> KYSKRIAWMKTTICDSLQLKDMIVEESFQYEKNKNLLEQFLSGEGLNKIFAYYQVQEQAQNDDIKDTGAQDPVLFFTTGDLEKIQDKAVWFLRITNPADDKKKASQQDGNDNDIIFGEITPNTVPMLNALMESVYSRQIDHIITEKIQFWGVAEEEQVLEFQQHSNKFSSEVREAINLMSPGTEHFKLDYEAISGLSESEKMQHYEMKFNEWINLISSQLNDDSEVRKDEKDAGPATELIYWRSRMQKITNWSEQLKSKDFQIVKASLQRHKNHDNQRPRGDESLSKLMMEYNRLDLLLTDKLNEAKDNVKYLTTLEKFIEPLYNGTPQQIIDTLPALMNAIKMIHTIARFYNTTDKMTGLFIKITNQMIKNCKDRILNKKDNGDNPSLYKMIWEQDPAELIEVLGSCIKLYCEYKKCYNDTKEKVADMPKGKTFDFSDAQIFGKFDTFVRRLQKLIEIFSNIQQFNALAKHNLEGMDVLTNKFKKIIDDFKKKGHNLLDTANNKFDRDWVEFNVEISHLDGELQNFIDNNFNRFRNIEYSLKLLHKFQSTIKRDSLKHNLTSRYNAILHNYATELDTIQRVFQDQKSNPPLVRNMPPEAGKIIWARHLFQKITGPINIFPENVINSTEIRRYYGSYNTLGKQLTIYEMWFYQDWVNKIEQSKAALQATLIVRHDENKKLYVNFDLEIMQLIREAKCLDRQGIEIPESARIILLQEDKFKTYYNELLYALKEYERINSKIKPICKNLLLPHIEDLDLKLRPGMVTLTWTSMNIESYLYYVHQGLKKLEQLIINVNDIIENRIENNLKTVSKVVLVHLPQDTKPLSLDSFVQLQEEYINSKTDFLTSKNVEVERAVDDLLQTIMLYPLDPHVDPVLPEETKRIKRYYFWYFYQALLNSTQNSLNAMKYRVCGKKIPGANTLQNLKPFFQVEVQLNGDKVTLNPSLQEIQKSINRAATAVLRCSKHLYNWDQQNKDSTDKATFYDMIACDKEIVKVILLLTGSIQGTKNKVNEFLSGFTKFEWLCKESIQESIKKFSKNGPTLQNYEDQLKKFSQIEEEIEKIVPTYKIGAMELMTHNICTSLSTWAKEWKLQYSQDLHKRARQLLDSLTEQTKMLSTKLSKPVKDIDSLGYVMETLEQIRKEQAEIDMKFNPVQEMYSLLDNYLPGGITDKDEMDARSLLRRNWDILIQQAEIKGKEYQHKQAIYLKELKQSIKDFTNQVSIFRRDYEKNGPMVEGISPAEAMERLRRFEDEYDVKYQMYKINARGENLFGLQNQKYPELEKTDAEIKNLNKLYNLYDSVIKNIQQFKEKSWQDVSKDDLAKMEEDAGKYGEQCSRLPKDLKEWQAYRDLKNYIDSLREQLPLIISLKKPSIMPRHWEKIKEITNTKLNYENPDQFYIEEIMGAKLLDFREDIEDITESADKQLKIRTGLDEINLYWNDMQFQFGIWGKRDVPCMLNGLIVGTILERLEEDQLQLSTFNSQRHVTPFKAEVENLIRTFSDVNDTLDMWVKVQKLWTSLEPVFTGGDIARQMPLQAKQFQGIDKNWMKIMEKAVETKKVIPCCQNDMLKDFLPDLNRKLEDCQKMLEAYLEGKRKKFPRFYFVSNPTLLKILSQGSEPTSIQEDFEKLFDAITKVTFESAKDKKNPALKQITQIQQVIGRNEENISLTGYYVKCEGNIEDWLKKLEQNMQQTLKDIASAAAQQVFQVGLKEFVSSQASQIALLGLQILWTSKVNEGLERLSRNERNAMDIKRNEIKEHMNILSSMCLEDLNGAVERTKVETLVTIQVHQKDISMDLKCKDVNDFEWQKQTRIAWKTDIDECIISITDWDSPYSYEFLGAKERLCITPLTDRCYITLAQAMSMYYGGAPAGPAGTGKTETVKDLGRTLGVFVVVTNCSDQHRYRDMAKIFKGLVQSGLWGCFDEFNRIDLEVLSVVAMQVESITTARKQHMKKFMFPEEEIEIELIPTVSYFITMNPGYAGRQELPENLKVLFRGVSMMVPDREIIIKVKLASVGYLQIDLLAKKFNVLYRLCEEQLSKQRHYDFGLRNILSVLRTAGNTKRQEIKSDEEMLLMRSLRDMNLSKLVADDIPLFNGLLADIFPKLKEVPKKLYPDVEKKIPEEINAESYLINTPSFQLKIIQLYETCLVRHGFMLVGPTGSGKSTIMKILTEVLTKLGSPHKIVIMNPKAITAEQMYGVKSEISDDWIPGVFSTIWAKSNNRALKHTTWITCDGPVDAIWIENLNTVLDDNKILTLANGERIAMTENCKVVFEVENLNNASPATVSRCGQVYVSPTDLGYEAVIEGWIRNRKASGRAEESDKLGNILRKYLINMRFIELQSKECKEPMMDTSPVISVINILNLLTGCLQYFVQTQRTLSEQEYEKFIVYSMAWAIGGIYEAQDRVRFHELLLAKNAPIPQKGKENETVFDYYVSQDYLDWKICSPEEWVPPQSLQFSQLLLPTLDSFRAEMLLNFILTQPKSHTCSNSALLIGGSGTAKTSSVLLYCNKFDPQKMLFKRTNFSSATSPFMFQSTIEAECDFKVGKEFAPPGNKMMTIFIDDMSMPFVNKWGDQITLELVRQLIETGGFYMLDKTQRGNQRKMKNLQYIGAMNHPGGGRNDIPNRLKRQFFIFNMILPLSIEGIYGPIIKHMFKQKYFSDSTYKVIESLTSATIALWNKVKSTMLPTPAKFHYVFNMRELSRIFKGILTCKKDTINDAPKSMKIKPELFLVGLWRHEAERVLADKLVNNKDKDTVMGYIQEVSLESFSQIENEILEKYSSEKTFLFCDFLRPDVINEDGIIEEEAPKIYEAIDSLTELRKRCNFLLSFYNDRNPSKKMPLVLFDDALKHLLRISRIIRQPRSSGLLVGVGGSGKQSLTRLAGFIGKNLIQQIIVTKTYSDKDLKEDIKKGFDDAGHLGKQVTFLMTDSEVKKEEFLEYINMVLSTGEIPNLLAKDEREVWLGDISQAYCKEKNLGNIDPPQSELWTYFVDRVRDNFHIMLCFSPVGQKFRERARKFPALFNECTIDWFLPWPEEALVSVAETFIKNFDKLDTKEETKQELMKHMGNVHLMVNEICDEYYQKMRRQVYVTPKSFLSYLNSYKTLYIEKYDELDQQEESFKIGLNKIQEATITINQMEISLKEEEIQLNEATEKTNQLLANLDKESKKANQKGEEVAATNKQCEIQAEQISKEKEEAERELEAALPALRRAQEAVDSIESKDIVELKANKKPLDIIKYIMNAVLVFFKARLIPIQIEERVFNKKEGKAVLFLKESYDESGIQTLGDMNFMKKLKEFEKDSINEETIELLEPYLNQSEDWFNDTFATKASKAAAGILKWAFAIYEYHQKSKIVKPKRIQVAIAEGRQAIALKELEKAREDLAQIQAYIKNLKDVYTKQMEEKNELEMKAAKTKKKINTARTLITSLSGEKDRWGKGAQDISDQKRKLVGNVSLSTAFISYCGPFNAEYRNKLAQQRFVVDMKKRGVPVTPGLELTSFLIDDATIGEWNLQGLPKDDLSIQNGIMVTNSARYPLFIDPQGQGQNWIRNKLSASIIPERCITTLSHPKFKDMFLKYCMESGLTLIVENIENEVDPMMDPVLERQIIVKGKTQFVNVAGTEMELSKEFKLFMTCRLANPSFSPELSAKTTIIDFTVTQSGLEQQLLGKVISKEQKALEDSLNQLLADVNQNQKDLQRLDKNLLERLINSQGNLLDDTELMDVLNNTKTQAKEVAAKLIDAEIKTKEINEKREQYRPVAIRGSAIYFTMIEVSLVNWMYNSSLEQFLKLFIESIDLSEKAQLPSNRVKNIISFLTFHVYRYVNRGLFEKDKITFILMMAFKILTTAGTISSGDVSLFLKSGDALDIKSERQKQISYLEDNQWLNILALSKHTFSGQTLPFFKELPDLISRSENQWRNWIDKNDPENFPIPDFAESINQEKEIGSFISLCLVRSLRNDRTLIATQNFISNVLGKEFTDPISYPIEGIWQESSNMDPVLFLLSAGADPTSSIDELAKKKKKFPCEKVSMGEGQERVARQVIMKGFVEGGWVILQNCHLGLKFMEEIETLVSPINQIHEDFRLWITCEQHPKFPLGLLQKTLKVTNEPPKGLKAGLYKTFTTIITQEFIDKVDHSNWRSLIFTICFLHSIVIERKKFGPLGWCVPYEYNYSDLEASLLYIEKYLTNLMSTPQPNSHNLPISMNVVRYMICEVQYGGRITDDLDRELFITYGETYLKDGIFGNDYFFYDIMVDGSGQKFKYRIPQNPSAELIKYQEYIAKVPTVDNPEVFGLHSNADLTFRLKESKEMINTVMETRPKDSSVGGGKTREEIVQDKAKDMLKNLPPDYNDVEVRELVSKLGGPNPKTSTERGMTVPLNIFLYQEVTRMQRVIGLVRKTLQDTILAIDGQIIMTPEILEAINAIYDAKVPNSWLYDPSGAEISWLLPNLGSWSTSLSDRNKQLNDWLRSGQRPILFWLTGFFNPQGFLTGMKQEVTRNHKKGDGKGGEAWSLDDVVYSTTVKEREKEKDIEQPPAEGVYIKGLYLEGCKWSKNGLDDSDPKKIFADLPILHVSAINKKKTNEQDRMSNTYLCPVYKYPKRTDKYLIFRVGLPCEGSNNPSHWKLRGVALLCST;> MGDHSQKDSPEDFIINRLSQALGIQKEKIKKSLETAQDDKGEVTNKDEFQGFIQQDNSTNILWVSGQSEKCTFYYGQLPPIDKFKKKGIAVIKLGLHKLTNENVAKDVVVVEITNNLLEHLNSVFNEIMSPVMQNPLNQQGWTDLVAKDLMEKFNNYVAQVYVLLGQIKGKTMLPLPSHKLTSSDTTPDKDKAHVFEGSIITWTKQIKNVLKLEPEQLLKYGNDPGPLAEIEFWQNKRDNLNLIDSQLKSVEVQNILHFLDNNKSTYTTPFTKLQAEVKKARLEANENYRYLFTLKDLFSKLQESQPSDFPTLYELFIPIMHTILLIYNKSKTYNQPPRLVVLIREICNAIISNAQAFVDKDTIFSLIDSKETTEACDKLQVTLDVCSKFKDAYFEYKAKAGGNWKLTSNALFVRLDSFLERCQDILHLTNTIVQFNKLEKIELGGTKGKTLTESIAQIFKEFEEAVQAFTSVSYDIMNIAEKKFDDDFYEFRSKIKELERRLASVITQGFDDYDTIYGRFKLLDNFEGLLTRPIIADELEKKHIVLLEMYKQDLKQVQSIFLEGKQFVDSMHENAPLFLNMPPIAGALTWCKSLRDRIQEPIEKLAQLGQGITEREEYKDVQKLYTSITKSIKDYEDQKILSWEKEVEDSSQDKLKQTLLCKDENDLIKVNFDPSLVRLLKEVKYFLLLRLEVPTTAKDIYTKAETYRTQIVALDMIVDNYNHIKTCLLPVEEPLVKKKIQDMEEEVKPGIEEIRWKSTNIDQFISKSKSIVDQLFETVNKMKDSLQKIHKSLANFNVKIIERKNRPMSPDDYDQFLKAIFSNKLTIVKDNGNQIQKLVKEVLDAVKADKKQNSWKNYNDYVNVIVIEGISTAIQTALLHLNEQINPVFIKRNDISPLFDIRLELGQSGIQFDPEIGESSNQLTVRNTIRNWINDFFNIAGTIQRLDTTMPGDFLQEIRSFFEIKQCLAMITQNLEWIENECNQFRARFDTYSYLWTEDEQISFNRFLDENEPKDEDGKGGDDDEGENTEKQNPLLKGCRAKIPNLDLFDEKITHLKAIQQEISRIKTPEDISWLRINLQPMKTALDARVTRWIRVYTDFLVNQFRTTQKNLLDFIEKTKDGIKKNPADHENLHDKKLLMSVMKVISDVKDVEPRREGIITRMKEMVTKLKKHNVPITEKGTDDPLQQIDNANSNFIEIYGRVFKVKADIIPLQAEETQNIKRDLDIFMKEVESFRKEFMQKLPFDYTESMGYENINNAYDTIMVYYHKLTAIEGRALEYNNLEKAFELQKSNYKQLKDCMNDLKNLKTMWDAIALIHFQYNDWKTKPWRQIKADILLDTNKTLGTQIKNLPKEIRNFKGYNVIVEKVKNMGTVLPLVSALHSEFMEDRHWSQLKQITGTVFDHNSLSFYFEDILALNLYKYENTVNEIVDVAQKEAKIEKKLKNIEQWWSKQVFEFTEYKETKTFASLDNMMEVLDQHSLDLMGMKSQGKYVEFFYDRVEDWREKLGRVDVVVNEWLKVQKNWKILYNIFLLSEDIRMQLPEDTKVFEGVDKEFKDMMSEVSANPSVVEACTIERRDVLVGWSQAIKKCEKALNDYLEQKKKSFPRFYFLSNQSLLTILSNGQNAPKVCEYLGDCFDGLKTLTFEPPANPAETSKVGIGMISKDDEKVPFSSKFICEGAVEHWLLNLEFRMRETLQEILEGAKNTADLWDSGDKPREEWVEGYNAQIALLTTTIVWTEDVGRAFEDLAGGSETAMKECQKLIEVRLENLIKKVRGDLHILERWKIINIITIDVHSRDVVEKFVIQKVSEAESFAWLSQLKFYWENKPDSDMHLRQTLRFPWEKDKNKNKCIIRIVDWFRFYSYEYIGNAIRLVITPLTDRCYITLTQALNLTMGGAPAGPAGTGKTETTKDLGRAIGIPVMVFNCSDQMNKDSMAQIFMGLSQSGAWGCFDEFNRISIEVLSVVSTQVKCVLDALKEKKTKFSFVEEGEIQLQDTVGFFITMNPGYAGRTELPENLKALFRSCAMVVPDLALICENMLMSEGFTMARVLSRKFVSLYMLSRELLSKQKHYDWGLRAVKSVLRQAGKLKRGDPDMPEDPLLMRALRDFNMPKIVTDDKVIFRRLIGDLFPKLDPPTKQNPELKKIVQDTTKKDMGLVAEELFVTKVVQLAEILEVRHCCFVIGPPGSGKTCVWKTLIKSYINSGEDAEYDTLNPKAVTSDELFGAYTKTKEWKNGVIAVIMKNQVKNEEKYKATHMHKWSVLDGDIDPEWIESLNTVMDDNKVLTLVSNDRIFLTPQMRLIFEISNLRNATPATVSRAGVLFINETDIGWMPYMNSWLERSQINILKQQKEMANMPEYPVIDDVAKSVFYRCFQSYFEQNIDVHDKNRVRHICPMVDIAMIQTICTILDALLIQHLPKLKQMKEEDEKQALEAFFIFAGLWAIGGPVGGGQDDSKDMKEFNTVWKGAAKVKFPEQGLCYDYYYDINENKWNTWKVEDYLPNDQPLFSKIYVATIHTTRLRYMIDIHLQRRKPILFIGSAGTGKTAVVRDYLNSTRPEQVSHKTINFSSFTDSLALQKNIESMVEKKNGRNYGSATNKVLICFIDDFNMPYVDKYGTQSPIQLLRLILDYGSIFNREQLEERKFLQDLLFFGCLNQKSGSFTVDLRLQRNFSVFSMYTPSSDVIKTIFGSILNAHLSTIDDKAQKMAFKLVEATYFTFDKILKNTTAFAPSAKRFHYQFNFRELARVCEGICRTTPGQYSGGDQGKLVRLWAHEMKRTFEDRFIANEHVEFFRRYLTEAISKCIGEFPETENPIAEPLIFTGFVAAHQGLDQQYTQCTIPVLKRVLDDKLEEYNEVKAQMNLVLFQQAMEHVSRICRILDMPGNNALLVGVGGSGKQSLCRLSTFINGFEIDQLVVTASFTINDLRNNLQEIYKKIAKPNSIARVFMITDSQIKEEQFLIPINDMLNSGWIFDLFPKEDMDSLVSGVRNEAKGEGVDVNNLTALTSYFLDKIRKNLKVVLCFSPVGDTMRIRSRKFPGIINNTSIDWFHPWPHEALIDVAFRFLEEIEFPTEEIRQSISLNMAKVHSSIDTANEKFLKLERRYNYTTPKSFLELIDFYKKLLTEKRETIQRQIQRYEMGLNILAETQNKVQGLQEELKVKMVEVNKQREETDILIEKVGKESALAEEEQTIANAEEEKTNVAAAEAEKISKEATEALAEALPALRSAEAAVDCLKKPHVTEMKNLGSPPAGVIVTARVVLILFNQGITLNDPDEKVWKKAVTFMNNPQAFIDKVKSFDGENIEPNIIEQSNKIIQDPSKKFNEKDMAGQSYAASKLCAWAVNIVTFNKIFKQVKPLQDAQKQANEILEEKKKELAIVKQRVAELNARVNSLKRQLEEAEARKMIVEQDAARCQSRLSAAENLVNGLAGENKRWTQNVKFLKENIKSMIGDSLLASAFVSYIGAFSAKLRLELWKNTWLPDIIEKGIPITEGIEPLKILTTEAIKSKWKNEGLPADPMSLENAAIITACARWPLIIDPQLQGSTWIRGKQGENLTTISLSQPKWLGALTSSISSGRAVLIEGIQQEIDATLDPLLQRAVKKNGNQLQLEIGGDPIDYDPNFKLFLMTKLINPHFRPEIAAQCTIINFIVTESGLEEQFIAMVVNIEKNELEMAKQDLVKKQNEYAVTLDKLESDLLQSLSEADPATILDNTELIQNLDKTKKTTIEITEQQQKAKVTEAEINIQREHYRVVAAEGSMLYFLVISLSVMDHMYQYSLESFITFFFKAINRTTVRDENRIPTLILNIRQTIYQWISRGLFEKHKLIFLTLIVFRLMQKKIIDVAYEVAEMDF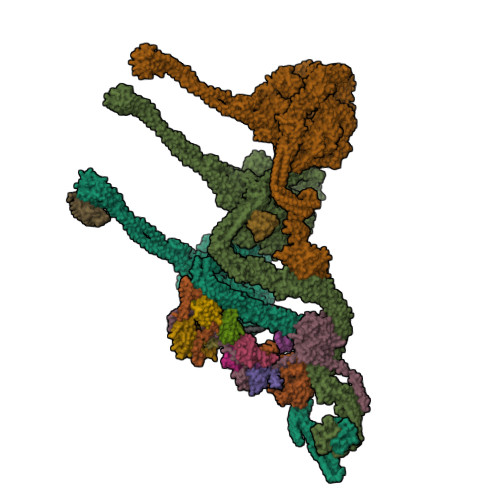LIKCPARPGVENTLDWLPNISWDQIQGLINLEEFRNFAHQLEKEAPNRFKDWYNELQPEDQKLPLDWKRLDSMPFKKLLVLRCLRPDRMTISLNNFIRAVLPQGDAFVEMDQKLAFSEILESVINEDAESTIPIFFILSPGSDPVKEVEKIAKKKRIEPGKNFFNIALGQGQDEIARRRIEEGNKEGHWVMLQNIHLMPTWLIELEKILDSYSGEAGGGNSEFRLFLSAEPSTGIPIGILDRSIKLTNEPPAGLKANMKRAWTYFSKEEIEDKDPKIKSILFALCFFHSTLIERRRFGPKGWNMSYPFNMGDLRDSYLVMNRYMEQNQGGKVPFNDLIYIFGEIMYGGHIVDDWDRRLCNSYLFNTMHEQLFDELELFPYIEGKGLSFKVPGQNPYEKYIEHIETSLKQETPLAYGLHPNAEIGFRTDQCKTLFNTLLELMPKEQSRDEKSSDIKSSNEMASDLIKQLLEDSELKNKIFNMEEIKNKIDAENKGPYQNVFLQEIEYMNALLSEIVKDLEEIGQGLSGLLTVSENMEMIIESIALSRVPASWQKLAYPSKRGLQSWLANLFQRIEQLNIFRDDPYSIPRVVMISRFFNPQSFLTAIMQVISRAKAYELNKLYIQTEITKRSIEEIEGAAKEGAYVYGFILEGARWDYQLGQLEESKPKEMFSVLPVTYCKAIPLPPEGKEDKSLYQCPVYKTEDRGNTYVFTAQLKTRFPPRKWILAGVAIIMDVEGVSD;> PLVWTQLKQTGTTQPTARSGHTIITVGKTHIMFGGLDNDKNNYKDGKIAPNNQVFTLKLTQNNCEWRQIACQGDVPLPRCYHASCAISADKMLVFGGSYTSNLRFNDTYILKTTSYQWSKPANQISGGEPKNAESKIGAPQPRYGHSATFFEGKVYIFGGHGGINYQRLAFNDLYVLETENFEWTRLEPKGNPPDPRGGHSAAMMANKPQLMIFGGWSFTSQYSNIMIYDIEKDEWVDPEIAHEIPKWNLSGIMAPSIPSWKYFIFGGSVGSFEEGGNRTNSRFVDDSFVLDIDTLSWSSINLEADETSKAVCKPRPRESASIFYDSGESRAIVFGGWANNWLNDLWALNVSTITGPPIFSIKPALGPLTGKTKVLIEGDGFKDTQNISVKFSGGKLEKEVNGTFVNEKEISCETPTFDYPRSVEVTVCMNKGDYTITKSAFTYNTKADKTIAYGPGLLTENLIGVQTTIVIQARNGSDEFVVTIRNPAKIKKEEEVKEGDKANTKNTIKEDEEEEGEDEEENKKKKEAEKNDLTGSAVMNYISKQLKDIQEFIENTKENIEIRNKNISELINVMINLEKVRVKNDDDVLTLDTVEEMLNFLKKKKDSDIKKCKKLQEEWKNLAKMAQAVKKDIQNPVKTESDKTKENIKKFEEITLKEYANSLKKESFFIYKTGVSESFKRIGEVKQKVDEFEVQLNQYEDFARIGSKKLMEQIRTDVSSVEKLWVRIEISEKTMDEYKKMKWGSINSMDMEDEIKKLRKALTDLRGIDKRSNAFIGITEELKKWATFLPLLGELKDPSMNSEDGRHWKKLKDLVKKEFDVSQELMLEIIWDLKLFDYKDGIEEITDQAKQELKMEKALKKIIDFWRDIEFELVQHKNTDIHTLKMSEENFETLEDHQLQINNMLLSKYVAYFEKEVEKWKYDLGSVYDVVQLLLEVQKTWSFLENLFEVKRELPNESAQFVGIDKDMKEIMQKGCDIKNCLKFCTIEGMLKRLENIQAQLKVCEKALNEFLDSKRRAFPRFYFVSVNDLLDILSNGNSPAKINRHMSKIFQAIDNLQLKEDSSGGRPTLKMISCVGTEEVDFSSPRLLQGKVESYLKDVIDTMIGTLKSVANSSFKNFQSMTRKEWLKSDPSQITLLVNNIIWSKAVEDCFLKLQSGDINAMKLFLDESIKQLTELIGMVQGDLSKPLRQKIMCLITIDTHSRDVVHRLINEHVRKAEEFQWQSQLKFYWVDNDAKIKIADARFVYNYEYLGNGPRLVITPLTDRIYVTATQALHLKMGCAPAGPAGTGKTETTKDLANALAKACYVFNCSSEMNYESMGNIYKGLASSGCWGCFDEFNRLLPEVLSVCSVQFKAVTDAIKQNVERFIIEGDEISLDPTCGVFITMNPGYLGRAELPEGLKALFRPITVVVPDLELICENMLMAEGFIEAKILAKKFVTLYMLCRDLLSKQLHYDWGLRAIKSVLVVAGGFKRSEPEIAEQALLMRALRDFNIPKIAFQDLYVFHGLLGDLFPGINIKPKKDLDFEKIITDVCIENKLDPDPEFVLKVVQLSELLAIRHCVFVMGPPGAGKSTTWKILAKAQDKTNKKTTLIDIDPKVVSTKDFYGYNLPSKEWKDGLFSKMLRSLAEQPDTNPKWICLDGDLDANWIESMNSVMDDNKILTLANNERIPLKPHMRALFEIRDLRFATPATVSRAGILYISDEVGYQWRSYVKSWIKQEFSQDQEMSKNLDTLFGKYVPDTLDHIKKHCRFLVPVSPISQVISICKSLQTLLKGDVKNLEYLFVYALIWAIGGALAEKDSIDYRKDFSTWWKGAWKTAVKFPSKGTIFDYYVDQSGDSSKFVEWSKRLENKEFDPQVETMGNITVNTIETLATTEFIKSYLMVKHPSLLIGNSGCGKTQLAKGILKEIVQAKPENYAYQLINFNYYTDSTYLQGQIEQTLEKKAGRQYGPPGKVQLIYFIDDLNMPQLDAYDTQTAIALLRQLADYGHFYDVSKLALKDIINTQVLAAMNPSAGSFFVNPRYQRHFWTISIPFPDNESLSLIYITFLNGHLKRFKSTIQEYSNIIVRASLMLHQAVTQNFRKTAINFHYEFNLRHMSNVFQGLLLSDPNKFTEPDKLIKLWIHECERTYGDRLVSTDNLKTYKENIFDIVKKSFSKFNFSRYFGNNPENLIYCNFIAGINSDRFYDQMPNNEMEKHISEALKEYNDNNAFMGLVLFEDAMKHVCRICRIVLPSSGHALLVGVGGSGKQSLSKLASFIMGYTTFSITISATYSMVDLRNDLQQLYFKCGPKEEGILFLFTEGQITNERFLVYINDLLSSGEIAELYTLDEKEAMINQVRAKVKGEGKPDTRENCWNWFIDQVKKNLHMAICFSPVGDMRRRARQFPALVNCTVIDWFQPWPYEALFNVAKSFLEPVDLGDDKVREAVVKFMPFSFTLVNDLGLKLLEQERRYAYTTPKSFLELISLFTNMLAQKRESLERNKERYETGLVKLKETAEQVAIIEVEVKEKQVEAEAKKKEADAFAEVVGREKDKVEKENSKATIEADKCGLIKQNVEAQKSSTQQDLDAAQPLVEQAKSALNSISKKDFQQAKSFASPPAGVPEVFAATIYLLAGYFNEAIEIDKNKKPKDVSWKSSLKLMKSPEEFMEKLLNFKDVVDANQVANVNIVKNQYLNMPSFTPEQMASKSAAAKGICSWVVNIVKYYDVIQDVEPKRKALKEATEQLEEATVKLNEVEEVVRKLNEELNKLKAENDKAIAERNAAISEAERCARRLNLAQRLVTALSSENERWGKSIIQLEDQLKLMVGDVLVASSFVSYSGPFNKKFRNIMINQNFMKFMKEHTIPMSPDPNPIKILTDESTIALWNKQKLPSDSVSIENGTILTNSARYPLMIDPQLQGITWIREKEKANNLKILRLGSKNINRDLELSIENGYSAIIENMNERIDAILMPIIARSFIKRGKNKIIKFAGKDLILHPNFKLFLHTKLSNPHYPPEIQAEAALINFTVTEAGLGDQLLSLVVARERPDLAKMKIELITQQNDFKIKLKDLEDELLYKLANAKGDILDDIELIENLEYSKKLSVEIAEKVAAAKITEAKINETSENYRPAASRGALFYFLLSDLSKVHSFYKYSLESFIVVINRAIDAISENKIYGKTTMMSPRSLKKRVDELIESLTYTAYQTTRRGLFESHKLIVAAMLCLRVLLRSEELNSDEVDHLIIGKVDVNPTPMPDALKSFLNDNIWAACKALETIHQFQGFCQSLETDVLQWKKWYSEEKAETADLPKAFKELSKFHRLLLLRALRPDRLPSALSQFVHDKMGERYIEQPPFNIFETFQETSKTVPIFFVLFPGVDPTPDVERVAATFDVSANNGRFINISMGQGQEDRAKKALFDCAQKGHWIMLQNVHLMQSWLYGLNGLEGFLESVFASPKTHPNFRVFISSEPPNVLLPLMQIIPESILQGSLKIANEAPQYLKANLRRAYNKFDQEFLDKCDKKPTEFKSCLFALCFFHSLMLGRKKFGTQGWSRVYNFNDGDLTICADVLYNYLSKYDQVPWDDLRYIFGEIMYGGHITDDWDRRTNRTYLKVLIRSELLQQNFNLAPQFKSPDPSKFDYEAYRKYIEEKLPIESPQMFGMHPNAEIGYLTQTCDQVFNTILEVQGGSSGGGASKKDDGVMVTLTDFKTRCPHDFNMLLIEEKVKEKTPYIVVCLQECERMNGLLKEIKTSLEDLRLGLTGALNMTDAMESLQQSLSFNKVPDTWEKKAYFSKKPLSSWFADLIERNIQLQEWCKELVTPTSLCISYLFNPMSYLTAIMQFTARAQGLPLDGITIQTNVTAMKGPEDVVNPAENGAYIHGLFLEGAAWEIGGQGQDGYLIEQKPKELHPKMPVINAVAVPLDKKKKNGQYDCPTYVTSARGQTFVFTANLNMESDDSDPNKWILSGTCMLMSDD;> LTAQELNEDMPSKMLEPKNPQAPKNITVYDYYTRKFKTDELVDQMIVHFSMDGDYIWKESNEYKTQEEIRDTKKALIKEAMRKQESEEPGANHDEEAIKQTLRNKFNYNTRECQTINPSIRERGVSTEPPPSDTICGNITQWEIFDAYYAEIMKDHQIENKKKKEVDQDKKQDQSMYSTSFKRCCKIMERMVVQNDQEDKYHDYRYYWSQGDNLEAGKNEGHLLPIWRFSNEKQRKKNVTSICWNPLYPDLFAVSLGSYDFTKQRMGLICLYSLKNTTHPEYAFNCEAGVMCLDFHPKSAALLAVGLYDGTVLVYDIRNKHKKPIYQSTVRNQKHTDPVWQVKWNPDTSKNYNFYSISSDGRVMNWILMKNKLEPEEVILLRLVGKNEEESTLIGLACGLCFDFNKFEPHIFLVGTEEGKIHKCSRAYSGQYQETYNGHLLAVYKVKWNNFHPRTFISASADWTVRIWDSKYTSQIICFDLSMMVVDAVWAPYSSTVFACATMDKVQVYDLNVDKLNKLAEQKIVKQPKLTNLSFNYKDPILLVGDSHGGVTLVKLSPNLCKSGPEIKQTEDKKAMEEFKNVKIEDYEREKMENL;> KEFNNPINFQDTETRYGGIQNQVVNINQYVQRNPNFIDLDNIAELSEHSVNTERVKTGDRGMSHKEGGWPGNVDPNEAQETGRFKKRIEKDTSFPQAVKDLKEGVEKCIYQNNQIDLLEEYFEGETSEHVVENLSSKTLMLFKDEKEICKRSVSEISWHPEGPTKVAVSYAIMRFQQMPEKMPTQAYVWDLLNPNSPEIKLMSPSAVTNISYNQKIPDQIGGGCYNGLLAVWDGRKGENPIMISPVENSHYEPVTHFHWLMSKTGSECVTTSTDGKVMWWDTRKFEAGPVEKLNIIEGLGENEEIIGGTALEYNVEAGPSKFLIGTESGSILTANKKLKKPVEITTRYGLDQGRHLGPVYSINRSNQNPKYFLSVGDWSCKIWVEDLKTPIIRTKYHGSYLSDGCWSPTRSGAFFLVRRDGWMDVWDYYYRQNEIAFSHKVSDSPLTCIKINQTGGAYHNSGKLCAIGDQDGTVTILELCDSLYTMQPKEKDIINEMFEREYRKEKNLETIKKQQELAKRQVQKDMGSQKEKWEKKKLEMIETAEASFHENLAKNPV;> NADDQLKQLSALEGANGYVIFNESGIPLKRHEKSISHEKAVHIAALVSDLWNVSKKVIQRDLKTPENDIEVIRLRTKHSYEYIITQSGDFTMLAIQLCGKAIEEAKKAAAAAAAAAVVQEENKEKEKK;> IYKTSKEIQKSDQRIIQQRVENSIINNQIYQKSLKRKTSKRKVRHQANKKNFQKEMSEVEDTLNRIKTHKTVLGYLIVNSEGGVVRGAFKDEEESKNIANSIPLLTKKARSVVRDLDPTNDLVFLRIQTKLNEIMVAPDDEFSLIVIQTKG;> SHLDKVQPVIKNSDMSVEMQKEVEEVAKKAIDYCNTDKEIATFIKDDFRSRYHGTWHCIVGRNFGSFVTFERSYYIYLYVGQLAILLFKTG;> KAVTDMDINELRKLMIGKAIINSSDMQGDLLQEAQDVIQSGIENNSAPVLNIEAACKYIKENLDKKFGPTWQCIIGEGYAYDVTVQNNTLLFMFYNGNLAVLIFKS;> QQYKTFMGARVLWPPECADDILEGAIRETQDALKKFEIAREGQKIAEHLKKYMDDHFDPYWHVFFGKNFGCQAVHNKNRFIYFYIEKTAFLMYQT;> HANEQIIDMPENSEMKSMKNDAFSQAKFAVENYKFENKISSHIKKFFDEKYGPNWHCVVGKHFNAYVSYDSKNFIFFYEGQLAILLYRKG;> MSDSDSDEGRVVEEPLPPHIIRFNDMAQHLLKKVIRQADVLIKENPQGLEKDIALNLVKFVKSQPEFKIGDGEWQCIIGKNFGCSLTFDANVLAFFDLLPSRKSILLFKSG;> MNHEPEVKATDMEEDMIKRVKEIAINAVKEYKQEKQIAHYIKYEFDKIDGYGWNCIVGRNFGSHIIHQTKKYIFFKINELCLLLWKA;> TDKEYISEEVQKAIDDSVKQVFGIKDDSSQVTITYNKDKVNLWTQQIIDYTIRGLNKLGKHFKYCVTAILQQTNHAGISVQITAYQDTATDGSLIQCYEINDIYAIVSVFAMAV;> RKREASLITLNYIKNRFYPSKIQKIIKELFEDRLKGVEYDPNNANQLSERLVLELREKIKRGKVPRYKIGVQVVFGEIKGQGLRIASKCLWDVQNDNYASYTYTSEKVYCTGIVFGCYFE;> TTTVTSEDHFMTFYNENNKKLIVVDVYPGWSGPCTAMYPTYNQLMISIDDFEKRIDILLLDQDKLVTYKNDKFHATCQPKFLFISEGKIIDEVLGTNIPVFIEKVNKYIPLS;> AKGTTCQKAIVNWEAANPGKNPSEAEEIKLIFQIPPIEKMDGPVLNTLTKCKKLSLSSNSIDKMISLNMLRNLEILSLSRNVIKKISGLEDIGGTLRQLWLSYNFIEKLDGLNNCSVLQTLYIGNNRIKNWEELDKLKDLPELENVLFYGNPIYEQVKEDPKLIVLKKLPTLKNVDGMIIDDSVLEKVKQIA;> MASEVMNLSEEDIQFCQKAFSDYDEDGLGAIKVSDLKLALENIGCSLSENDLFKMISEVDEKNTGLIKFSDFLNIYYKQKYANLGDDDQDLVDAFVAMGGNADTTGSVDANRLIQIVKEEFEMTIDIVGLIREIDKDGSGEIEYEEFKLL>[2x]MAATVDTMSEEVKRLIALYELTPHPASGGWFRETYRSDVQVE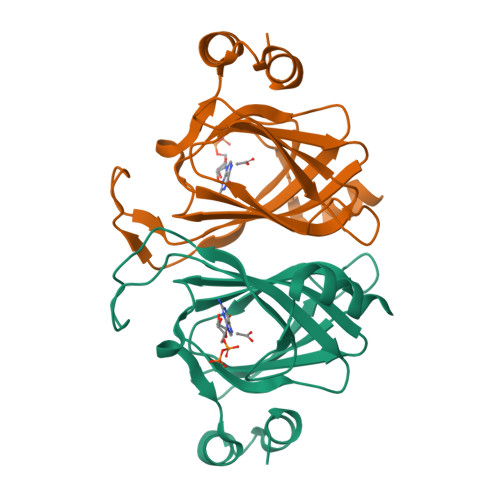AEGFDGKRSVLTMIYYLMQAGQPDPFHRVKSDETFVHNLGGSMKIHMIHPDGSYSCSILGNPLEHPEARHQVVVPRRVWFAQEVDGYCLASVLVAPGFDFKDFSLGKREELIKEYPQHRDVIMRCTSSDP>[2x]DENASAAEQVNKTIIGIDPGSGIMSLTDKAMKDYDLNDWTLISASSAAMTATLKKSYDRKKPIIITGWTPHWMFSRYKLKYLDDPKQSYGSAEEIHTITRKGFSKEQPNAAKLLSQFKWTQDEMGEIMIKVEEGEKPAKVAAEYVNKHKDQIAEWTKGVQKVKGD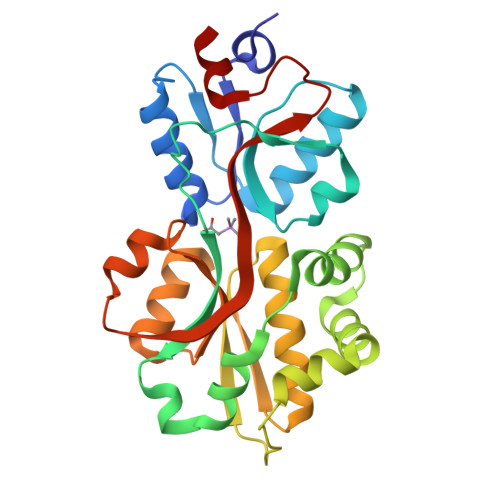KINLAYVAWDSEIASTNVIGKVLEDLGYEVTLTQVEAGPMWTAIATGSADASLSAWLPNTHKAYAAKYKGKYDDIGTSMTGVKMGLVVPQYMKNVNSIEDLKK N-{3-[(5R)-3-amino-2,5-dimethyl-1,1-dioxido-5,6-dihydro-2H-1,2,4-thiadiazin-5-yl]-4-fluorophenyl}-5-fluoropyridine-2-carboxamide | C17 H17 F2 N5 O3 S | 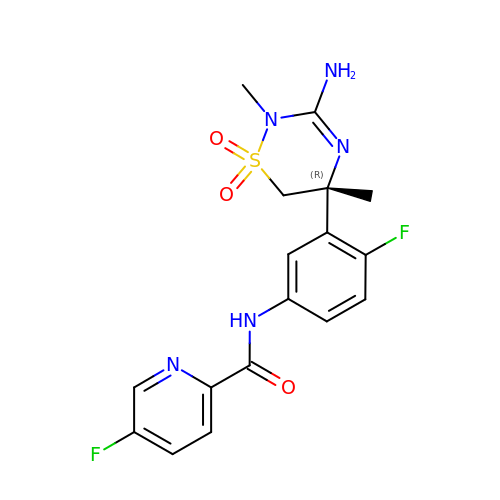YHYKUSGACIYRML-KRWDZBQOSA-N LMW-PTP is a well-characterised phospho-tyrosine specific PTP, widely expressed in human tissues and conserved through evolution. The ligand-binding interface of LMW-PTP comprises the active site P-loop, the adjacent DPYY-loop (D-loop) and the variable region or variable loop. The catalytic residues C12 (nucleophile) and R18 (phosphate binding) are located in the P-loop, and D129 (general acid/base) in the D-loop. We demonstrate here that minimal re-design of LMW-PTP, by mutating only two residues, is sufficient to introduce new enzymatic activity towards four different phosphoinositide (PI) substrates.

Mammalian lipid phosphatases (PTEN, INPP4A, and INPP4B) have a conserved lysine in the P-loop that is important for substrate binding. In the LMW-PTP-WT this lysine corresponds to an isoleucine in position 16 of and thus we used the LMW-PTP-I16K mutant as starting template for RosettaDesign in DS2. In order to assess the actual impact of the designed mutations on the protein structure, we determined the crystal structures of the I16K and L13R-I16K mutants at 1.8Å and 2.0Å resolution respectively. In both cases, the structures are similar to the WT enzyme with overall root-mean deviations (RMSDs) of 0.288 Å and 0.265 Å respectively. There are no structural distortions in main chain of the P-loop or the variable region, thus the mutations introduced do not alter the tertiary structure of the protein, consistent with a catalytically active enzyme. However, in both structures, the side chain of W49 is in the open position, away from the active site, thus confirming the flexibility of this side chain as suggested from the kinetics characterisation. Importantly, the crystal structures of the K16 and R13-K16 designs show that mutations introduced in the new enzymes do not alter the 3D structure of the protein or the position of the catalytic residues. This ensures that the catalytic mechanism remains unaltered in the mutants.

> AEQATKSVLFVCLGNKCRSPIAEAVFRKLVTDQNISENWVIDSGAVSDWNVGRSPDPRAVSCLRNHGIHTAHKARQITKEDFATFDYILCMDESNLRDLNRKSNQVKTCKAKIELLGSYDPQKQLIIEDPYYGNDSDFETVYQQCVRCCRAFLEKAH> ADPQKLDDVDPLVTTNFGKIRGIKKELNNEILGPVIQFLGVPYAAPPTGEHRFQPPEPPSPWSDIRNATQFAPVCPQNIIDGRLPEVMLPVWFTNNLDVVSSYVQDQSEDCLYLNIYVPTEDDIRDSGGPKPVMVYIHGGSYMEGTGNLYDGSVLASYGNVIVITVNYRLGVLGFLSTGDQAAKGNYGLLDLIQALRWTSENIGFFGGDPLRITVFGSGAGGSCVNLLTLSHYSEKGLFQRAIAQSGTALSSWAVSFQPAKYARILATKVGCNVSDTVELVECLQKKPYKELVDQDVQPARYHIAFGPVIDGDVIPDDPQILMEQGEFLNYDIMLGVNQGEGLKFVENIVDSDDGVSASDFDFAVSNFVDNLYGYPEGKDVLRETIKFMYTDWADRHNPETRRKTLLALFTDHQWVAPAVATADLHSNFGSPTYFYAFYHHCQTDQVPAWADAAHGDEVPYVLGIPMIGPTELFPCNFSKNDVMLSAVVMTYWTNFAKTGDPNQPVPQDTKFIHTK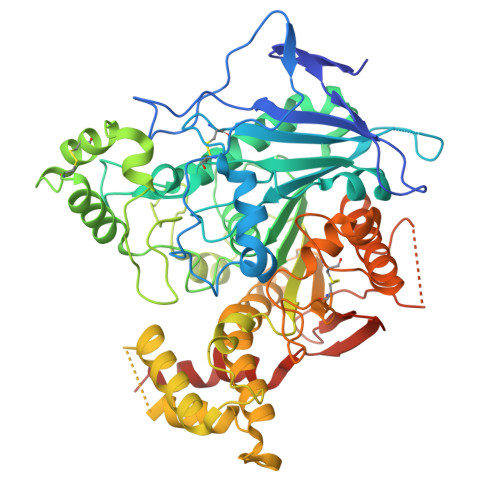PNRFEEVAWTRYSQKDQLYLHIGLKPRVKEHYRANKVNLWLELVPHLHNLNDHHHHHH>[4x]MGGSSGGGVSYRSGGESDVELEDYEVDDFRDGIVESRGNRFNPLTNFLGLDFAGGSGGKFTVINGIRDISRGSIVHPDNRWYKAWTMFILIWALYSSFFTPLEFGFFRGLPENLFILDIAGQIAFLVDIVLTFFVAYRDSRTYRMIYKRSSIALRYLKSTFIIDLLACMPWDIIYKAAGEKEEVRYLLLIRLYRVHRVILFFHKMEKDIRINYLFTRIVKLIFVELYCTHTAACIFYYLATTLPASQEGYTWIGSLKLGDYSYSKFREIDLWTRYTTSMYFAVVTMATVGYGDIHA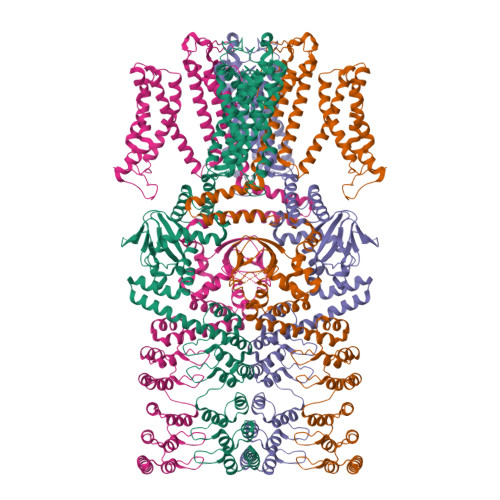VNMREMIFAMVYISFDMILGAYLIGNMTALIVKGSKTERFRDKMADIMRYMNRNKLGRNIRGQITGHLRLQYESSYTEAAVLQDIPVSIRAKIAQTLYLPYIEKVPLFRGCSSEFINQIVIRLHEEFFLPGEVIMEQGSVVDQLYFVCHGVLEEIGITKDGSEEIVAVLQPDHSFGEISILCNIPQPYTVRVAELCRILRLDKQSFMNILEIFFHDGRRILNNLLEGKESNVRIKQLESDITFHISKQEAELALKLNSAAFYGDLYQLKSLIRAGGDPNKTDYDGRSPLHLAASRGYEDITLYLIQESVDVNIKDKLGSTPLLEAIKNGNDRVAALLVKEGATLNIENAGTFLCTVVAKGDSDFLKRLLSNGIDPNSKDYDHRTPLHVAASEGFYVLAIQLVEASANVLAKDRWGNTPLDEALGCGNKMLIKLLEDAKNSQISSFPSGSKEPKDKVYKKKCTVYFSHPGDSKEKRRRGIVLWVPRSIEELIRTAKEQLNVPEASCVLSEDEAKIIDVDLISDGQKLYLAVET> DSIMKILLIGDSGVGKSCLLVRFVEDKFNPSFITT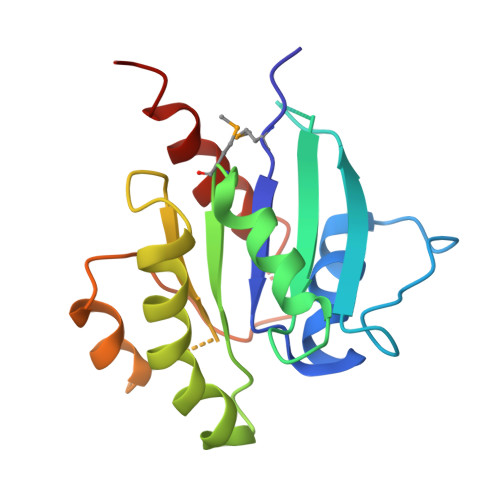IGIDFKIKTVDINGKKVKLQLWDTAGQERFRTITTAYYRGAMGIILVYDVTDERTFTNIKQWFKTVNEHANDEAQLLLVGNKSDMETRVVTADQGEALAKELGIPFIESSAKNDDNVNEIFFTLAKLIQEKIDSN>[2x]AGALWEIEKELFTKLPAPSSAINSHLQPAKPKVPQKKPSKWDPPAEFKVDLSTAVSYNDIGDINWKNLQQFKGIERSEKGTEGLFFVETESGVFIVKRSTNIESETFCSLLCMRLGLHAPKVRVVSSNSEEGTNM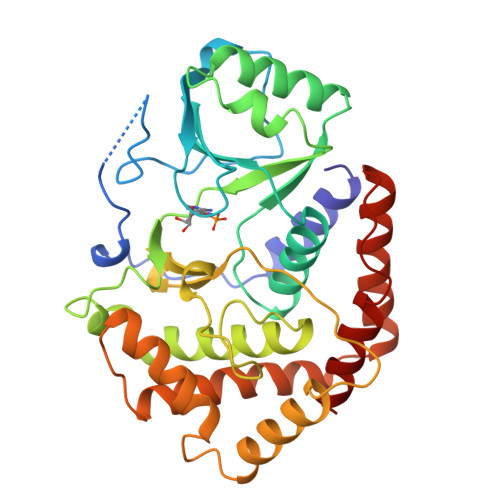LECLAAIDKSFRVITTLANQANILLMELVRGITLNKLTTTSAPEVLTKSTMQQLGSLMALDVIVNNSDRLPIAWTNEGNLDNIMLSERGATVVPIDSKIIPLDASHPHGERVRELLRTLIAHPGHESSQFHSIRDIITLYTGYDVGTEGSISMQEGFLATVRECASFDLDAFERELLSWQESLQKCHNLSISPQAIPFILRMLRIFH> MSSEKEELRERLVKIVVENAKRKGDDTEEAREAAREAFELVREAAERAGIDSSEVLELAIRLIKEVVENAQREGYDISEAARAAAEAFKRVAEAAKRAGITSSEVLELAIRLIKEVVENAQREGYDISEAARAAAEAFKRVAEAAKRAGITSSETLKRAIEEIRKR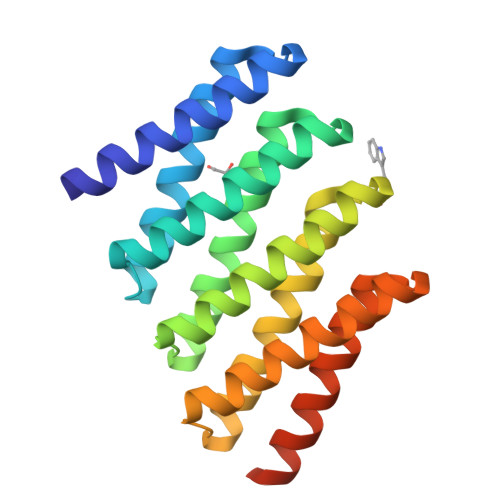VEEAQREGNDISEAARQAAEEFRKKAEELKRRGDGWLEHHHHHH>[2x]MRRSVYFCGSIRGGREDQALYARIVSRLRRYGKVLTEHVADAELEPLGEEAAGGDQFIHEQNLNWLQQADVVVAEVTQPSLGVGYELGRAVALGKPILCL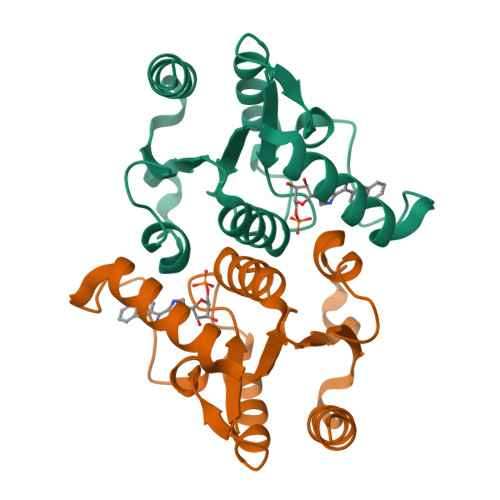FRPQSGRVLSAMIRGAADGSRFQVWDYAEGEVETMLDRYFEAYLVEHHHHHH>[6x]MNAEINPLHAYFKLPNTVSLVAGSSEGETPLNAFDGALLNAGIGNVNLIRISAIMPPEAEIVPLPKLPMGALVPTAYGYIISDVPGETISAAISVAIPKD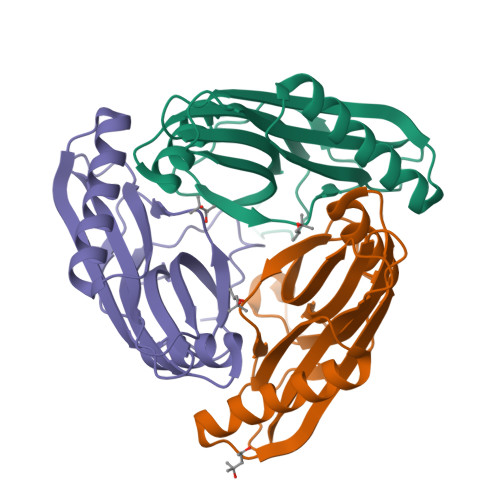KSLCGLIMEYEGKCSKKEAEKTVREMAKIGFEMRGWELDRIESIAVEHTVEKLGCAFAAAALWYK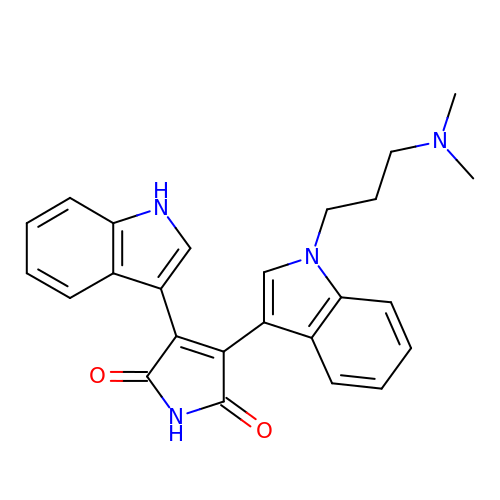3-{1-[3-(DIMETHYLAMINO)PROPYL]-1H-INDOL-3-YL}-4-(1H-INDOL-3-YL)-1H-PYRROLE-2,5-DIONE | C25 H24 N4 O2 | QMGUOJYZJKLOLH-UHFFFAOYSA-N>PSTRDYEIQRERIELGRCIGEGQFGDVHQGIYMSPENPALAVAIKTCKNCTSDSVREKFLQEALTMRQFDHPHIVKLIGVITENPVWIIMELCTLGELRSFLQVRKYSLDLASLILYAYQLSTALAYLESKRFVHRDIAARNVLVSSNDCVKLGDFGLSRYMEDSTYYKASKGKLPIKWMAPESINFRRFTSASDVWMFGVCMWEILMHGVKPFQGVKNNDVIG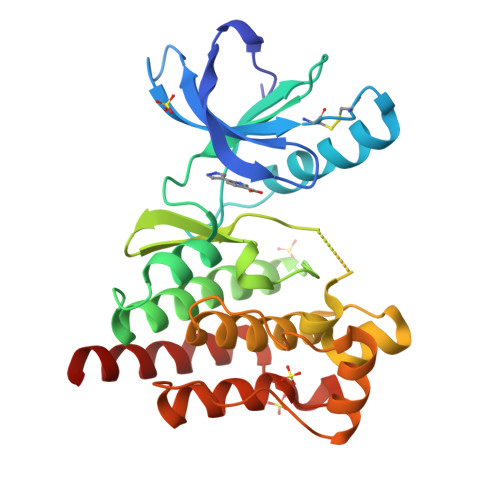RIENGERLPMPPNCPPTLYSLMTKCWAYDPSRRPRFTELKAQLSTILEEEKAQ[2x]> MAIDEIKSRGYLLVGLSADFPPFEFVDENGNIVGFDVDLAKEIARRLGVELKIVDMTFDGLIPSLLTKKIDVIISGMTITEERKKVVAFSDPYFDAGQVIVVRKDSDF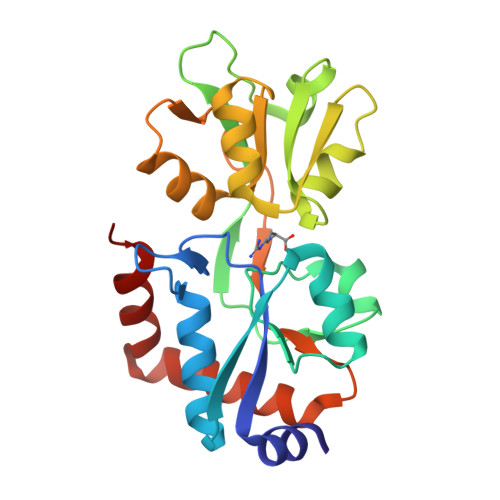RPKTYEDLVGKTVAVQIGTTGDIEVSKYDGIKVVRFDKFTDAFLELKRGRADAVVLDSATARAFVAKNPDLVISSGVLSSEQYGIAVRKEDTDLLEFINSVLRELKKSGKYDVLIEKWFSE N-[(2E)-3-(biphenyl-4-yl)prop-2-enoyl]-beta-D-glucopyranosylamine | C21 H23 N 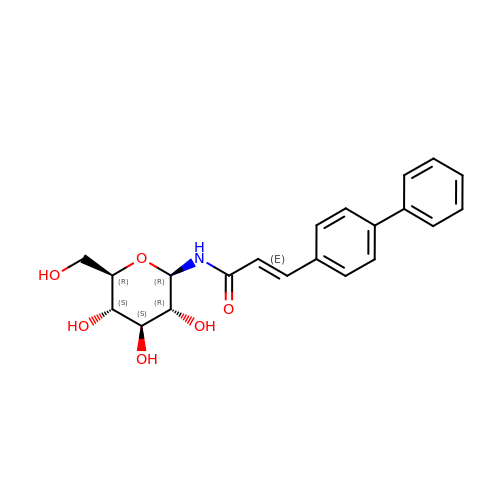O6 | BXIQZJVUHNZTDW-KLXRIHHNSA-N>[2x]GAMDPMIVLGLEGTAHTISCGIIDESRILAMESSMYRPKTGGIRPLDAAVHHSEVIDTVISRALEKAKISIHDIDLIGFSMGPGLAPSLRVTATAARTISVLTGKPIIGVNHPLGHIEIGRRVTGAIDPVMLYVSGGNTQVIAHVNGRYRVLGETLDIGIGNMIDKFAREAGIPFPGGPEIEKLAMKGTKLLDLPYSVKGMDTAFSGILTAALQYLKTGQAIEDISYSIQETA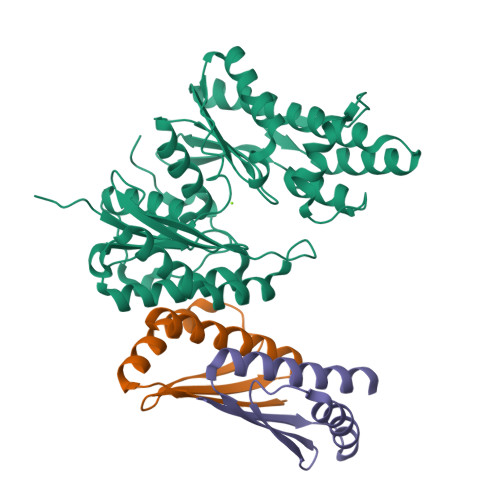FAMLVEVLERALYVSGKDEILMAGGVALNRRLRDMVTNMAREAGIRSYLTDREYCMDNGIMIAQAALLMYKSGVRMSVEETAVNPRFRIDEVDAPWITDAS;>[4x]GAMDPMKAKRVQAKIEMEFPSEDVAKVVYEAVLYEHLSVPYRRSEIDFKLEGKKIILDIKATDSSALRGTVNSYLRWIKAAIDVIEV> MSELFGVLKSNAGRIILKDPSATSKDVKAYIDSVINTCKNGSITKKAELDEITVDGLDANQVWWQVKLVLDSIDGDLIQGIQELKDVVTPSHNLSDGSTLNSSSGEESELEEAESVFKEKQMLSADVSEIEEQSNDSLSENDEEPSMDDEKTSAEAAREEFAEEKRISSGQDERHSSPDPYGINDKFFDLEKFNRDTLAAEDSNEASEGSEDEDIDYFQDMPSDDEEEEAIYYEDFFDKPTKEPVKKHSDVKDPKEDEELDEEEHDSAMDKVKLDLFADEEDEPNAEGVGEASDKNLSSFEKQQIEIRKQIEQLENEAVAEKKWSLKGEVKAKDRPEDALLTEELEFDRTAKPVPVITSEVTESLEDMIRRRIQDSNFDDLQRRTLLDITRKSQRPQFELSDVKSSKSLAEIYEDDYTRAEDESALSEELQKAHSEISELYANLVYKLDVLSSVHFVPKPASTSLEIRVETPTISMEDAQPLYMSNASSLAPQEIYNVGKAEKDGEIRLKNGVAMSKEELTREDKNRLRRALKRKRSKANLPNVNKRSKRNDVVDTLSKAKNITVINQKGEKKDVSGKTKKSRSGPDSTNIKL;> MSNGHVKFDADESQASASAVTDRQDDVLVISKKDKEVHSSSDEESDDDDAPQEEGLHSGKSEVESQITQREEAIRLEQSQLRSKRRKQNELYAKQKKSVNETEVTDEVIAELPEELLKNIDQKDEGSTQYSSSRHVTFDKLDESDENEEALAKAIKTKKRKTLKNLRKDSVKRGKFRVQLLSTTQDSKTLPPKKESSIIRSKDRWLNRKALNKG;> MTQSLGIEQYKLSVVSGGKPALNNLSSVTGNKNIARLSQDQRNYIIPFNNQIKVYSVETRQCVKTLKFANNSLLSGIFLQEEENNESIVKILLGDITVPQQEDAHLITVFTNNGHVIVLNYKGKLVESPKHFKISLADEKLANVFHSEGNYRILTTFKDPSQKAHNSLQSYRLYALTFDDAKKQFEVAHQAEWHNVILSNISSNGKLLAHMCKDVSTKDHEHKSISVVSLFDDSVNLSFPLGSILSSQTQSLSYNTRYVSSMAIDNMGQQLAVGFASGVISIVSLADLQIRLLKWHIDSVLSLSFSHDGSYLLSGGWEKVMSLWQLETNSQQFLPRLNGIIIDCQVLGPQGNYYSLILQMTENNSNSDYQFLLLNASDLTSKLSINGPLPVFNSTIKHIQQPISAMNTKNSNSITSLNHSKKKQSRKLIKSRRQDFTTNVEINPINKNLYFPHISAVQIFDFYKNEQVNYQYLTSGVNNSMGKVRFELNLQDPIITDLKFTKDGQWMITYEIEYPPNDLLSSKDLTHILKFWTKNDNETNWNLKTKVINPHGISVPITKILPSPRSVNNSQGCLTADNNGGLKFWSFDSHESNWCLKKISLPNFNHFSNSVSLAWSQDGSLIFHGFDDKLQILDFDTFKKFESLENTKTVSEFTLDSEIQTVKLINDTNLIVATRTTLNAINLLRGQVINSFDLYPFVNGVYKNGHMDRLITCDERTGNIALVINQQLTDLDGVPTINYKSRIIIFDSDLSTKLGNFTHHEYISWIGWNYDTDFIFLDIESTLGVVGTXXXXXXXXXXXXXXNDEDEEDIALEFINGEKKDKLVNMNSFTSMFDNIQNVQMDTFFDRVMKVLT;> MSTARPRIITSKAPLLPQQTTPEQRYWRQYTSAQLVKEHNSVTHISFNPQHPHDFAVTSSTRVQIFSSRTRQVIKTFSRFKDVVYSASFRSDGKLLCAGDATGLVSVYDSYNPRTILLSINASTHPTHVTKFHTQDNKILATASDDRVTRLWDISNAYEPQLELTGATDYVRTLSFIPAAPHLVATGSYDGLIRLYDTRSSGSTPIYSLNHDQPVENVIAVSPTQIVSCGGNNFKVWDLTSNKKLYERGNFNKAVTCLDYVENFDSPMQSALIASSLDGHVKVFDPLDNFQVKFGWKFSGPVLSCAVSPSTAQGNRHLVAGLSSGLLAIRTKKKEKRSSDKENAPASFNKNAKSNNFQRMMRGSEYQGDQEHIIHNDKVRSQRRMRAFERNINQFKWSEALDNAFVPGMAKELTLTVLQELRKRGKVRVALYGRDESTLEPLLNWCLKGIEDVRSASIVADWVAVVLELYGNTLESSPVLQELMIDLKTKVRHEIHKSKEAQRIEGMLQLLTS;> XXXXXXXXXXXXXXXXXXXXXXXXXXXXXXXXXXXDHLSKIFLTISKSITQNPWNEENLLPLWLKWLLTLKSGELNSIKDKHTKKNCKHLKSALRSSEEILPVLLGIQGRLEMLRRQAKLREDLAQLSMQEGEDDEIEVIEHSNVISNPLQDQASPVEKLEPDSIVYANGESDEFVDASEYKD;> MDSPVLQSAYDPSGQYLCYVTVALDKQRVGVQPTQRATSSGVDTVWNENFLYLEDSKLKVTCLKWVNLASSDTVAIILGMNNGEIWLYSVLANEVTYKFTTGNSYEIKDIDLMGNQLWCIDSSDAFYQFDLLQFKLLQHFRINNCVQLNKLTIVPAGDSVAQLLVASHSISLIDIEEKKVVMTFPGHVSPVSTLQVITNEFFISGAEGDRFLNVYDIHSGMTKCVLVAESDIKELSHSGQADSIAVTTEDGSLEIFVDPLVSSSTKKRGNKSKKSSKKIQIVSKDGRKVPIYNAFINKDLLNVSWLQNATMPYFKNLQWREIPNEYTVEISLNWNNKNKSADRDLHGKDLASATNYVEGNARVTSGDNFKHVDDAIKSWERELTSLEQEQAKPPQANELLTETFGDKLESSTVARISGKKTNLKGSNLKTATTTGTVTVILSQALQSNDHSLLETVLNNRDERVIRDTIFRLKPALAVILLERLAERIARQTHRQGPLNVWVKWCLIIHGGYLVSIPNLMSTLSSLHSTLKRRSDLLPRLLALDARLDCTINKFKTLNYEAGDIHSSEPVVEEDEDDVEYNEELDDAGLIEDGEESYGSEEEEEGDSDNEEEQKHTSSKQDGRLETEQSDGEEEAGYSDVEME;> MSSLSDQLAQVASNNATVALDRKRRQKLHSASLIYNSKTAATQDYDFIFENASKALEELSQIEPKFAIFSRTLFSESSISLDRNVQTKEEIKDLDNAINAYLLLASSKWYLAPTLHATEWLVRRFQIHVKNTEMLLLSTLNYYQTPVFKRILSIIKLPPLFNCLSNFVRSEKPPTALTMIKLFNDMDFLKLYTSYLDQCIKHNATYTNQLLFTTCCFINVVAFNSNNDEKLNQLVPILLEISAKLLASKSKDCQIAAHTILVVFATALPLKKTIILAAMETILSNLDAKEAKHSALLTICKLFQTLKGQGNVDQLPSKIFKLFDSKFDTVSILTFLDKEDKPVCDKFITSYTRSIARYDRSKLNIILSLLKKIRLERYEVRLIITDLIYLSEILEDKSQLVELFEYFISINEDLVLKCLKSLGLTGELFEIRLTTSLFTNADVNTDIVKQLSDPVETTKKDTASFQTFLDKHSELINTTNVSMLTETGERYKKVLSLFTEAIGKGYKASSFLTSFFTTLESRITFLLRVTISPAAPTALKLISLNNIAKYINSIEKEVNIFTLVPCLICALRDASIKVRTGVKKILSLIAKRPSTKHYFLSDKLYGENVTIPMLNPKDSEAWLSGFLNEYVTENYDISRILTPKRNEKVFLMFWANQALLIPSPYAKTVLLDNLNKSPTYASSYSSLFEEFISHYLENRSSWEKSCIANKTNFEHFERSLVNLVSPKEKQSFMIDFVLSALNSDYEQLANIAAERLISIFASLNNAQKLKIVQNIVDSSSNVESSYDTVGVLQSLPLDSDIFVSILNQNSISNEMDQTDFSKRRRRRSSTSKNAFLKEEVSQLAELHLRKLTIILEALDKVRNVGSEKLLFTLLSLLSDLETLDQDGGLPVLYAQETLISCTLNTITYLKEHGCTELTNVRADILVSAIRNSASPQVQNKLLLVIGSLATLSSEVILHSVMPIFTFMGAHSIRQDDEFTTKVVERTILTVVPALIKNSKGNEKEEMEFLLLSFTTALQHVPRHRRVKLFSTLIKTLDPVKALGSFLFLIAQQYSSALVNFKIGEARILIEFIKALLVDLHVNEELSGLNDLLDIIKLLTSSKSSSEKKKSLESRVLFSNGVLNFSESEFLTFMNNTFEFINKITEETDQDYYDVRRNLRLKVYSVLLDETSDKKLIRNIREEFGTLLEGVLFFINSVELTFSCITSQENEEASDSETSLSDHTTEIKEILFKVLGNVLQILPVDEFVNAVLPLLSTSTNEDIRYHLTLVIGSKFELEGSEAIPIVNNVMKVLLDRMPLESKSVVISQVILNTMTALVSKYGKKLEGSILTQALTLATEKVSSDMTEVKISSLALITNCVQVLGVKSIAFYPKIVPPSIKLFDASLADSSNPLKEQLQVAILLLFAGLIKRIPSFLMSNILDVLHVIYFSREVDSSIRLSVISLIIENIDLKEVLKVLFRIWSTEIATSNDTVAVSLFLSTLESTVENIDKKSATSQSPIFFKLLLSLFEFRSISSFDNNTISRIEASVHEISNSYVLKMNDKVFRPLFVILVRWAFDGEGVTNAGITETERLLAFFKFFNKLQENLRGIITSYFTYLLEPVDMLLKRFISKDMENVNLRRLVINSLTSSLKFDRDEYWKSTSRFELISVSLVNQLSNIENSIGKYLVKAIGALASNNSGVDEHNQILNKLIVEHMKASCSSNEKLWAIRAMKLIYSKIGESWLVLLPQLVPVIAELLEDDDEEIEREVRTGLVKVVENVLGEPFDRYLD;> MSSSLLSVLKEKSRSLKIRNKPVKMTSQERMIVHRCRFVDFTPATITSLAFSHKSNINKLTPSDLRLAIGRSNGNIEIWNPRNNWFQEMVIEGGKDRSIEGLCWSNVNGESLRLFSIGGSTVVTEWDLATGLPLRNYDCNSGVIWSISINDSQDKLSVGCDNGTVVLIDISGGPGVLEHDTILMRQEARVLTLAWKKDDFVIGGCSDGRIRIWSAQKNDENMGRLLHTMKVDKAKKESTLVWSVIYLPRTDQIASGDSTGSIKFWDFQFATLNQSFKAHDADVLCLTTDTDNNYVFSAGVDRKIFQFSQNTNKSQKNNRWVNSSNRLLHGNDIRAICAYQSKGADFLVSGGVEKTLVINSLTSFSNGNYRKMPTVEPYSKNVLVNKEQRLVVSWSESTVKIWTMGTDSSTEQNYKLVCKLTLKDDQNISTCSLSPDGQVLVVGRPSTTKVFHLQPVGNKLKVTKLDNDLLLRTSTKLVKFIDNSKIVICSCEDDVFIVDLESEEDEKPQEVELLEVTSTKSSIKVPYINRINHLEVDQNIAVISRGCGVVDILDLKARISKPLARLNNFITAVHINTSRKSVVVITADNKIYEFNMNLNSEAENEDSESVLTQWSKNNTDNLPKEWKTLKENCVGIFSDIENSSRLWFWGATWISRIDFDVDFPINKXXXXXXXXXXXXXXHFFFTDKYKPLLFVDLISSNELAIIERNPLTFHSKQKAFIQPKLVF;> MKSDFKFSNLLGTVYRQGNITFSDDGKQLLSPVGNRVSVFDLINNKSFTFEYEHRKNIAAIDLNKQGTLLISIDEDGRAILVNFKARNVLHHFNFKEKCSAVKFSPDGRLFALASGRFLQIWKTPDVNKDRQFAPFVRHRVHAGHFQDITSLTWSQDSRFILTTSKDLSAKIWSVDSEEKNLAATTFNGHRDYVMGAFFSHDQEKIYTVSKDGAVFVWEFTKRPSDDDDNESEDDDKQEEVDISKYSWRITKKHFFYANQAKVKCVTFHPATRLLAVGFTSGEFRLYDLPDFTLIQQLSMGQNPVNTVSVNQTGEWLAFGSSKLGQLLVYEWQSESYILKQQGHFDSTNSLAYSPDGSRVVTASEDGKIKVWDITSGFCLATFEEHTSSVTAVQFAKRGQVMFSSSLDGTVRAWDLIRYRNFRTFTGTERIQFNCLAVDPSGEVVCAGSLDNFDIHVWSVQTGQLLDALSGHEGPVSCLSFSQENSVLASASWDKTIRIWSIFGRSQQVEPIEVYSDVLALSMRPDGKEVAVSTLKGQISIFNIEDAKQVGNIDCRKDIISGRFNQDRFTAKNSERSKFFTTIHYSFDGMAIVAGGNNNSICLYDVPNEVLLKRFIVSRNMALNGTLEFLNSKKMTEAGSLDLIDDAGENSDLEDRIDNSLPGSQRGGDLSTRKMRPEVRVTSVQFSPTANAFAAASTEGLLIYSTNDTILFDPFDLDVDVTPHSTVEALREKQFLNALVMAFRLNEEYLINKVYEAIPIKEIPLVASNIPAIYLPRILKFIGDFAIESQHIEFNLIWIKALLSASGGYINEHKYLFSTAMRSIQRFIVRVAKEVVNTTTDNKYTYRFLVSTDGSMEDGAADDDEVLLKDDADEDNEENEENDVVMESDDEEGWIGFNGKDNKLPLSNENDSSDEEENEKELP;> MVKSYQRFEQAAAFGVIASNANCVWIPASSGNSNGSGPGQLITSALEDVNIWDIKTGDLVSKLSDGLPPGASDARGAKPAECTYLEAHKDTDLLAVGYADGVIKVWDLMSKTVLLNFNGHKAAITLLQFDGTGTRLISGSKDSNIIVWDLVGEVGLYKLRSHKDSITGFWCQGEDWLISTSKDGMIKLWDLKTHQCIETHIAHTGECWGLAVKDDLLITTGTDSQVKIWKLDIENDKMGGKLTEMGIFEKQSKQRGLKIEFITNSSDKTSFFYIQNADKTIETFRIRKEEEIARGLKKREKRLKEXXXXXXXXXXYSSFILHPFQTIRSLYKIKSASWTTVSSSKLELVLTTSSNTIEYYSIPYEKRDPTSPAPLKTHTIELQGQRTDVRSIDISDDNKLLATASNGSLKIWNIKTHKCIRTFECGYALTCKFLPGGLLVILGTRNGELQLFDLASSSLLDTIEDAHDAAIWSLDLTSDGKRLVTGSADKTVKFWDFKVENSLVPGTKNKFLPVLKLHHDTTLELTDDILCVRVSPDDRYLAISLLDNTVKVFFLDSMKFYLSLYGHKLPVLSIDISFDSKMIITSSADKNIKIWGLDFGDCHKSLFAHQDSIMNVKFLPQSHNFFSCSKDAVVKYWDGEKFECIQKLYAHQSEVWALAVATDGGFVVSSSHDHSIRIWEETEDXXXXXXXXXXXXXXXXXXXXXXXXXSGVHKQTLESLKAGERLMEALDLGIAEIEGLEAYNRDMKLWQRKKLGEAPIKPQGNAVLIAVNKTPEQYIMDTLLRIRMSQLEDALMVMPFSYVLKFLKFIDTVMQNKTLLHSHLPLICKNLFFIIKFNHKELVSQKNEELKLQINRVKTELRSALKSTEDDLGFNVQGLKFVKQQWNLRHNYEFVDEYDQQEKESNSARKRVFGTVI;> MTMATTAMNVSVPPPDEEEQLLAKFVFGDTTDLQENLAKFNADFIFNEQEMDVEDQEDEGSESDNSEEDEAQNGELDHVNNDQLFFVDDGGNEDSQDKNEDTMDVDDEDDSSSDDYSEDSEEAAWIDSDDEKIKVPILVTNKTKKLRTSYNESKINGVHYINRLRSQFEKIYPRPKWVDDESDSELDDEEDDEEEGSNNVINGDINALTKILSTTYNYKDTLSNSKLLPPKKLDIVRLKDANASHPSHSAIQSLSFHPSKPLLLTGGYDKTLRIYHIDGKTNHLVTSLHLVGSPIQTCTFYTSLSNQNQQNIFTAGRRRYMHSWDLSLENLTHSQTAKIEKFSRLYGHESTQRSFENFKVAHLQNSQTNSVHGIVLLQGNNGWINILHSTSGLWLMGCKIEGVITDFCIDYQPISRGKFRTILIAVNAYGEVWEFDLNKNGHVIRRWKDQGGVGITKIQVGGGTTTTCPALQISKIKQNRWLAVGSESGFVNLYDRNNAMTSSTPTPVAALDQLTTTISNLQFSPDGQILCMASRAVKDALRLVHLPSCSVFSNWPTSGTPLGKVTSVAFSPSGGLLAVGNEQGKVRLWKLNHY;> MSIDLKKRKVEEDVRSRGKNSKIFSPFRIIGNVSNGVPFATGTLGSTFYIVTCVGKTFQIYDANTLHLLFVSEKETPSSIVALSAHFHYVYAAYENKVGIYKRGIEEHLLELETDANVEHLCIFGDYLCASTDDNSIFIYKKSDPQDKYPSEFYTKLTVTEIQGGEIVSLQHLATYLNKLTVVTKSNVLLFNVRTGKLVFTSNEFPDQITTAEPAPVLDIIALGTVTGEVIMFNMRKGKRIRTIKIPQSRISSLSFRTDGSSHLSVGTSSGDLIFYDLDRRSRIHVLKNIHRESYGGVTQATFLNGQPIIVTSGGDNSLKEYVFDPSLSQGSGDVVVQPPRYLRSRGGHSQPPSYIAFADSQSHFMLSASKDRSLWSFSLRKDAQSQEMSQRLHKKQDGGRVGGSTIKSKFPEIVALAIENARIGEWENIITAHKDEKFARTWDMRNKRVGRWTFDTTDDGFVKSVAMSQCGNFGFIGSSNGSITIYNMQSGILRKKYKLHKRAVTGISLDGMNRKMVSCGLDGIVGFYDFNKSTLLGKLKLDAPITAMVYHRSSDLFALALDDLSIVVIDAVTQRVVRQLWGHSNRITAFDFSPEGRWIVSASLDSTIRTWDLPTGGCIDGIIVDNVATNVKFSPNGDLLATTHVTGNGICIWTNRAQFKTVSTRTIDESEFARMALPSTSVRGNDSMLSGALESNGGEDLNDIDFNTYTSLEQIDKELLTLSIGPRSKMNTLLHLDVIRKRSKPKEAPKKSEKLPFFLQLSGEKVGDEASVREGIAHETPEEIHRRDQEAQKKLDAEEQMNKFKVTGRLGFESHFTKQLREGSQSKDYSSLLATLINFSPAAVDLEIRSLNSFEPFDEIVWFIDALTQGLKSNKNFELYETFMSLLFKAHGDVIHANNKNQDIASALQNWEDVHKKEDRLDDLVKFCMGVAAFVTTA;> MKIKTIKRSADDYVPVKSTQESQMPRNLNPELHPFERAREYTKALNATKLERMFAKPFVGQLGYGHRDGVYAIAKNYGSLNKLATGSADGVIKYWNMSTREEFVSFKAHYGLVTGLCVTQPRFHDKKPDLKSQNFMLSCSDDKTVKLWSINVDDYSNKNSSDNDSVTNEEGLIRTFDGESAFQGIDSHRENSTFATGGAKIHLWDVNRLKPVSDLSWGADNITSLKFNQNETDILASTGSDNSIVLYDLRTNSPTQKIVQTMRTNAICWNPMEAFNFVTANEDHNAYYYDMRNLSRSLNVFKDHVSAVMDVDFSPTGDEIVTGSYDKSIRIYKTNHGHSREIYHTKRMQHVFQVKYSMDSKYIISGSDDGNVRLWRSKAWERSNVKTTREKNKLEYDEKLKERFRHMPEIKRISRHRHVPQVIKKAQEIKNIELSSIKRREANERRTRKDMPYISERKKQIVGTVHKYEDSGRDRKRRKEDDKRDTQEK;> MGHKKNGHRRQIKERENQNKFERSTYTNNAKNNHTQTKDKKLRAGLKKIDEQYKKAVSSAAATDYLLPESNGYLEPENELEKTFKVQQSEIKSSVDVSTANKALDLSLKEFGPYHIKYAKNGTHLLITGRKGHVASMDWRKGQLRAELFLNETCHSATYLQNEQYFAVAQKKYTFIYDHEGTELHRLKQHIEARHLDFLPYHYLLVTAGETGWLKYHDVSTGQLVSELRTKAGPTMAMAQNPWNAVMHLGHSNGTVSLWSPSMPEPLVKLLSARGPVNSIAIDRSGYYMATTGADRSMKIWDIRNFKQLHSVESLPTPGTNVSISDTGLLALSRGPHVTLWKDALKLSGDSKPCFGSMGGNPHRNTPYMSHLFAGNKVENLGFVPFEDLLGVGHQTGITNLIVPGAGEANYDALELNPFETKKQRQEQEVRTLLNKLPADTITLDPNSIGSVDKRSSTIRLNAKDLAQTTMDANNKAKTNSDIPDVKPDVKGKNSGLRSFLRKKTQNVIDERKLRVQKQLDKEKNIRKRNHQIKQGLISEDHKDVIEEALSRFG;> MVRKLKHHEQKLLKKVDFLEWKQDQGHRDTQVMRTYHIQNREDYHKYNRICGDIRRLANKLSLLPPTDPFRRKHEQLLLDKLYAMGVLTTKSKISDLENKVTVSAICRRRLPVIMHRLKMAETIQDAVKFIEQGHVRVGPNLINDPAYLVTRNMEDYVTWVDNSKIKKTLLRYRNQIDDFDFS;> MAPIEYLLFEEPTGYAVFKVKLQQDDIGSRLKEVQEQINDFGAFTKLIELVSFAPFKGAAEALENANDISEGLVSESLKAILDLNLPKASSKKKNITLAISDKNLGPSIKEEFPYVDCISNELAQDLIRGVRLHGEKLFKGLQSGDLERAQLGLGHAYSRAKVKFSVQKNDNHIIQAIALLDQLDKDINTFAMRVKEWYGWHFPELAKLVPDNYTFAKLVLFIKDKAXXXXXXXXXXXXXXXXXXXXXXXXXXSETDMENVCVFAQRVASLADYRRQLYDYLCEKMHTVAPNLSELIGEVIGARLISHAGSLTNLSKQAASTVQILGAEKALFRALKTKGNTPKYGLIYHSGFISKASAKNKGRISRYLANKCSMASRIDNYSEEPSNVFGSVLKKQVEQRLEFYNTGKPTLKNELAIQEAMELYNKDKPAAEVEETKEKESSKKRKLEDDDEEKKEKKEKKSKKEKKEKKEKKDKKEKKDKKEKKDKKKKSKD;>[2x]MSFRPGSRGGSRGGSRGGFGGRGGSRGGARGGSRGGFGGRGGSRGGARGGSRGGFGGRGGSRGGARGGSRGGRGGAAGGARGGAKVVIEPHRHAGVYIARGKEDLLVTKNMAPGESVYGEKRISVEEPSKEDGVPPTKVEYRVWNPFRSKLAAGIMGGLDELFIAPGKKVLYLGAASGTSVSHVSDVVGPEGVVYAVEFSHRPGRELISMAKKRPNIIPIIEDARHPQKYRMLIGMVDCVFADVAQPDQARIIALNSHMFLKDQGGVVISIKANCIDSTVDAETVFAREVQKLREERIKPLEQLTLEPYERDHCIVVGRYMRSGLKK;>[2x]MSAPNPKAFPLADAALTQQILDVVQQAANLRQLKKGANEATKTLNRGISEFIIMAADCEPIEILLHLPLLCEDKNVPYVFVPSRVALGRACGVSRPVIAASITTNDASAIKTQIYAVKDKIETLLI;> MSDVTQQKKRKRSKGEVNPSKPTVDEEITDPSSNEDEQLEVSDEEDALESEEEFEGENPADKRRRLAKQYLENLKSEANDILTDNRNAEEKDLNNLKERTIDEYNNFDAGDLDKDIIASRLKEDVAEQQGRVFRYFGDKLLISEAKQSFTRVGENNLTCISCFQPVLNKYTFEESSNGDKNKGRLFAYTVSKDLQLTKYDITDFSKRPKKLKYAKGGAKYIPTSKHEYENTTEGHYDEILTVAASPDGKYVVTGGRDRKLIVWSTESLSPVKVIPTKDRRGEVLSLAFRKNSDQLYASCADFKIRTYSINQFSQLEILYGHHDIVEDISALAMERCVTVGARDRTAMLWKIPDETRLTFRGGDEPQKLLRRWMKENAKEGEDGEVKYPDESEAPLFFCEGSIDVVSMVDDFHFITGSDNGNICLWSLAKKKPIFTERIAHGILPEPSFNDISGETDEELRKRQLQGKKLLQPFWITSLYAIPYSNVFISGSWSGSLKVWKISDNLRSFELLGELSGAKGVVTKIQVVESGKHGKEKFRILASIAKEHRLGRWIANVSGARNGIYSAVIDQTGF;> MGKAKKTRKFGLVKRTLNTKKDQRLKKNQENIKTKEDPELTRNIPQVSSALFFQYNQAIKPPYQVLIDTNFINFSIQKKVDIVRGMMDCLLAKCNPLITDCVMAELEKLGPKYRIALKLARDPRIKRLSCSHKGTYADDCLVHRVLQHKCYIVATNDAGLKQRIRKIPGIPLMSVGGHAYVIEKLPDVF

The first structurally defined particle that assembles co-transcriptionally is therefore the small subunit processome, a giant precursor of the small subunit. The particle containing the 5’ ETS region and its associated 26 unique polypeptides was termed the 5’ ETS particle. Recent structural studies of the fully assembled SSU processome have shown that the 5’ ETS and its associated multi-protein complexes UtpA, UtpB and U3 snoRNP form a scaffold for the assembly of individual rRNA domains, thus further highlighting the central role of the 5’ ETS. Conformational switches within the 5’ ETS RNP contribute to the regulated formation of the SSU processome by inhibiting binding of late assembly factors that are associated with the compaction of the SSU processome upon completed transcription of the 18S rRNA.

Although individual rRNA domains are flexible and functionally independent modules, we observed the 5’ ETS RNP as the unifying and stable structural entity in each of these reconstructions. Multi-protein complexes UtpA and UtpB as well as the U3 snoRNP constitute the major components of this assembly. Additional proteins such as Utp7, Sof1, and Imp3 with its associated segment of Mpp10 are clearly visible. Compared with the SSU processome, the most dramatic conformational changes occur within the UtpB complex. This complex adopts a conformation that reconfigures its tetramerization module as well as the tandem β-propellers of Utp12 and Utp13 into a compacted state. As a result of this large conformational change, several binding sites for other assembly factors are disrupted, such as the bipartite binding site of the late factor Pno1, the binding sites for the C-terminal region of Mpp10, the Rcl1•Bms1 complex, several ribosomal proteins, and the 18S pre-rRNA. Continuous density extending from helices VII and VIII of the 5’ ETS is for the first time observed between Sof1 and Utp7. This density corresponds to the base of helix IX of the 5’ ETS and contains the A0 cleavage site. In the 5’ ETS RNP, an RNA linker and helix IX sterically prevent the association of the late binding factor Utp14, which binds in the same region in the SSU processome after A0 cleavage or RNA remodeling.> SNAMTKVLFVKANNRPAEQAVSVKLYEAFLASYKEAHPNDTVVELDLYKEELPYVGVDMINGTFKAGKGFDLTEEEAKAVAVADKYLNQFLEADKVVFGFPLWNLTIPAVLHTYIDYLNRAGKTFKYTPEGP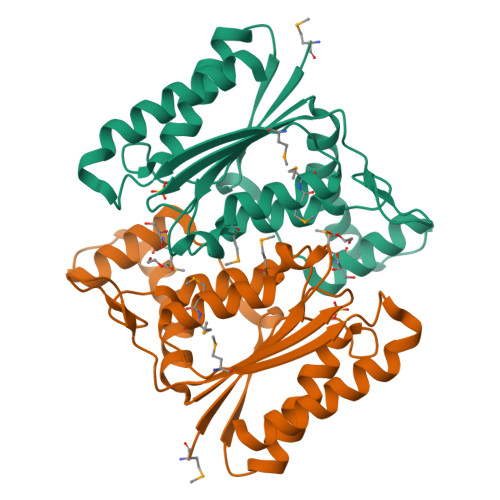VGLIGDKKIALLNARGGVYSEGPAAEVEMAVKYVASMMGFFGATNMETVVIEGHNQFPDKAEEIITAGLEEAAKVANKF> AHHHHHHGSLEIRTKVGEICISKVWLTDEQINKLFDRFKGDYQVVNAECADKVIFATIIAIKAVKEGRSI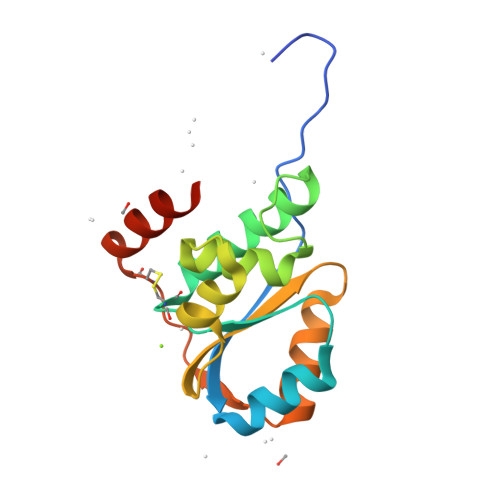AKTVPGEILVRLSGNRQIKEAIKKVGAKEGENYIVTFGENASALLQKILSTLEIKELELERCDLEYAKKAFEDIAIIEAL>[6x]GAMGSGVLPRPCRVLVLLNPRGGKGKALQLFRSHVQPLLAEAEISFTLMLTERRNHARELVRSEELGRWDALVVMSGDGLMHEVVN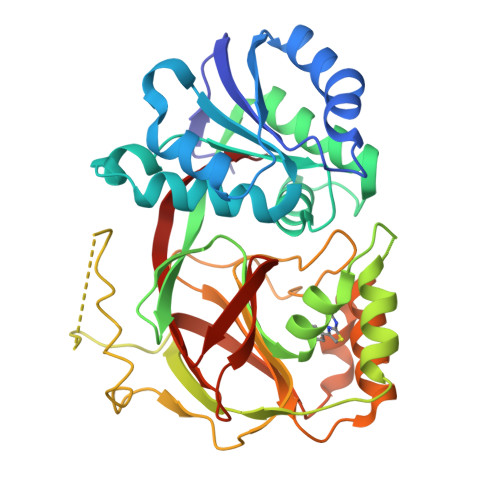GLMERPDWETAIQKPLCSLPAGSGNALAASLNHYAGYEQVTNEDLLTNCTLLLCRRLLSPMNLLSLHTASGLRLFSVLSLAWGFIADVDLESEKYRRLGEMRFTLGTFLRLAALRTYRGRLAYLPVGRVGSKTPASPVVVQQGPVDAHLVPLEEPVPSHWTVVPDEDFVLVLALLHSHLGSEMFAAPMGRCAAGVMHLFYVRAGVSRAMLLRLFLAMEKGRHMEYECPYLVYVPVVAFRLEPKDGKGVFAVDGELMVSEAVQGQVHPNYFWMVSG4-(4-ethylcyclohexyl)morpholine 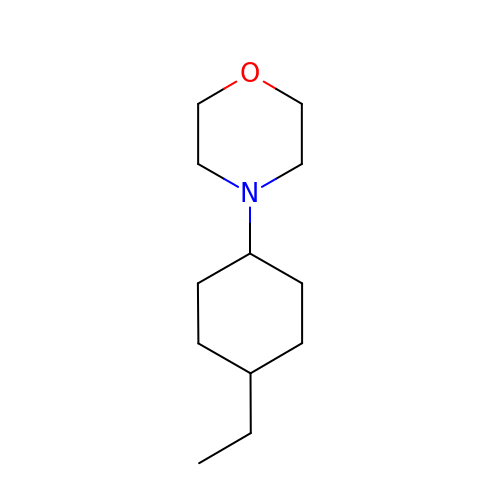| C12 H23 N O | UXPACUHPXVTRQE-HAQNSBGRSA-N> DWISFSHMSSDTDHFPIKSWFRCEQKAASRSYRTLGDMSHPQGIYEVRAAITRLISLTRGVKCRPEQMIIGAGTQVLMQLLTELLPKEAVYAMEEPGYRRMYQLLKNAGKQVKTIMLDEKGMSIAEITRQQPDVLVTTPSHQFPSGTIMPVSRRIQLLNWAAEEPRRYIIEDDYDSEFTYDVDSIPALQSLDRFQNVIYMGTFSKSLLPGLRI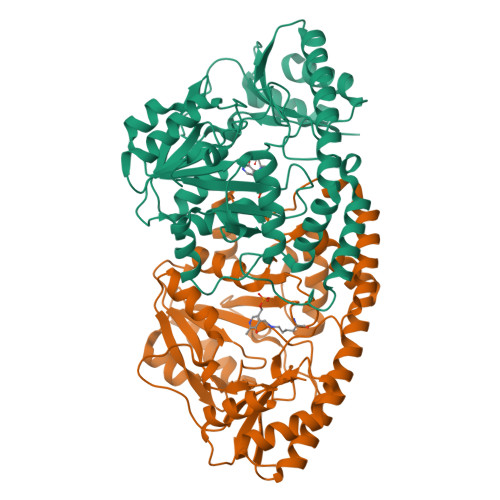SYMVLPPELLRAYKQRGYDLQTCSSLTQLTLQEFIESGEYQKHIKKMKQHYKEKRERLITALEAEFSGEVTVKGANAGLHFVTEFDTRRTEQDILSHAAGLQLEIFGMSRFNLKENKRQTGRPALIIGFARLKEEDIQEGVQRLFKAVYG;> DWISFSHMSSDTDHFPIKSWFRCEQKAASRSYRTLGDMSHPQGIYEVRAAITRLISLTRGVKCRPEQMIIGAGTQVLMQLLTELLPKEAVYAMEEPGYRRMYQLLKNAGKQVKTIMLDEKGMSIAEITRQQPDVLVTTPSHQFPSGTIMPVSRRIQLLNWAAEEPRRYIIEDDYDSEFTYDVDSIPALQSLDRFQNVIYMGTFSKSLLPGLRISYMVLPPELLRAYKQRGYDLQTCSSLTQLTLQEFIESGEYQKHIKKMKQHYKEKRERLITALEAEFSGEVTVKGANAGLHFVTEFDTRRTEQDILSHAAGLQLEIFGMSRFNLKENKRQTGRPALIIGFARLKEEDIQEGVQRLFKAVYGHR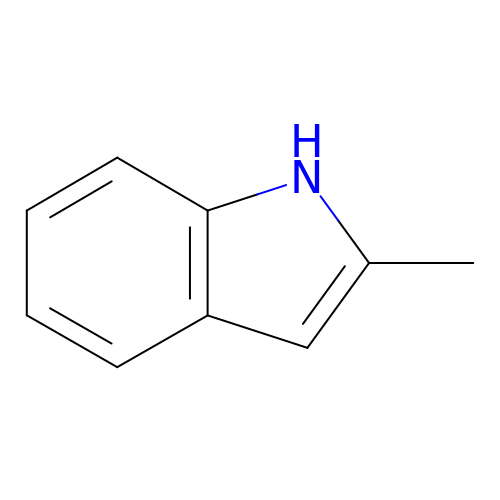2-METHYL-1H-INDOLE | C9 H9 N | BHNHHSOHWZKFOX-UHFFFAOYSA-N> HHHHHHPEIVDTCSLASPASVCRTKHLHLRCSVDFTRRTLTGTAALTVQSQEDNLRSLVLDTKDLTIEKVVINGQEVKYALGERQSYKGSPMEISLPIALSKNQEIVIEISFETSPKSSALQWLTPEQTSGKEHPYLFSQCQAIHCRAILPCQDTPSVKLTYTAEVSVPKELVALMSAIRDGETPDPEDPSRKIYKFIQKVPIPCYLIALVVGALESRQIGPRTLVWSEKEQVEKSAYEFSETESMLKIAEDLGGPYVWGQYDLLVLPPSFPYGGMENPCLTFVTPTLLAGDKSLSNVIAHEISHSWTG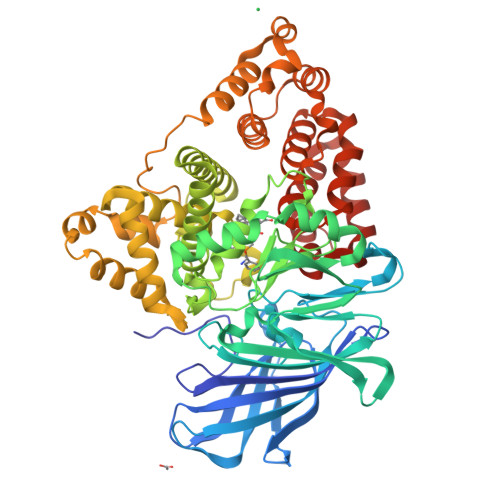NLVTNKTWDHFWLNEGHTVYLERHICGRLFGEKFRHFNALGGWGELQNSVKTFGETHPFTKLVVDLTDIDPDVAYSSVPYEKGFALLFYLEQLLGGPEIFLGFLKAYVEKFSYKSITTDDWKDFLYSYFKDKVDVLNQVDWNAWLYSPGLPPIKPNYDMTLTNACIALSQRWITAKEDDLNSFNATDLKDLSSHQLNEFLAQTLQRAPLPLGHIKRMQEVYNFNAINNSEIRFRWLRLCIQSKWEDAIPLALKMATEQGRMKFTRPLFKDLAAFDKSHDQAVRTYQEHKASMHPVTAMLVGKDLKVD> GSGGGDDMSNAGDFLNDNAVEIPSFSKGIINDDEDDEDLMMASGRPRQRSHILEDDENSVDISMLKTGSSLLKEEEEDGQEGSIHNLPLVTSQRPFYDGPMPTPRQKPFQSGSTPLHLTHRFMVWNSIGIIRCYNDEQDNAIDVEFHDTSIHHATHLSNTLNYTIADLSHEAILLACESTDELASKLHCLHFSSWDSSKEWIIDLPQNEDIEAICLGQGWAAAATSALLLRLFTIGGVQKEVFSLAGPVVSMAGHGEQLFIVYHRGTGFDGDQCLGVQLLELGKKKKQILHGDPLPLTRKSYLAWIGFSAEGTPCYVDSEGIVRMLNRGLGNTWTPICNTREHCKGKSDHYWVVGIHENPQQLRCIPCKGSRFPPTLPRPAVAILSFKLPYCQIATEKGQMEEQFWRSVIFHNHLDYLAKNGYEYEESTKNQATKEQQELLMKMLALSCKLEREFRCVELADLMTQNAVNLAIKYASRSRKLILAQKLSELAVEKAAELTAT

Ctf4 orthologues have been identified in various eukaryotic organisms, including fission yeast (Mcl1), Drosophila (Ctf4) and humans (acidic and nucleoplasmic DNA-binding protein; AND-1), suggesting that its functional role has been conserved throughout evolution. AND-1 clearly shares some or possibly all the functions of its yeast counterpart in maintaining genome stability and establishing sister chromatid cohesion. This is a likely consequence of its sequence similarity with Ctf4 (21% identity and 36% similarity over 722 out of 1129 aligned residues) and their shared domain structure, comprising an N-terminal β-propeller domain and a C-terminal SepB domain, the latter being responsible for trimerization and for interactions with proteins harbouring a Ctf4-interacting peptide (CIP) motif. Here, we show that the SepB domain of AND-1 is a structural orthologue of yeast Ctf4, that it exists in a trimeric form and that it binds to Pol α/primase, like its yeast orthologue Ctf4.

To investigate further the structural basis for the interaction of AND-1 with Pol α, we determined the crystal structure of amino acids 329–826 of human AND-1, comprising its SepB domain, which correspond to the region of Ctf4 (Ctf4CTD) that we had previously characterized. Despite the low sequence identity (17%, based on structure superposition), the AND-1 SepB structure bears a remarkable resemblance to that of yeast Ctf4CTD, with the same tertiary structure comprising a six-bladed β-propeller fused to a C-terminal bundle of five α-helices, and an RMSD value of 1.8 Å over 305 Cα positions. In the AND-1 structure, the trimeric arrangement of protomers seen for Ctf4 arises from crystallographic symmetry, and it was confirmed by size-exclusion chromatography multi-angle laser light scattering measurements. Indeed, inspection of the putative binding site for its client proteins, based on structural homology with the Ctf4CTD structure, highlights a solvent-exposed hydrophobic patch formed by M766, A770, A792, L795 and Y799. The pulldown experiments showed a clear interaction of Pol α148–171 with AND-1336–826, which was not observed for the double alanine mutant. Together, these findings indicate that AND-1336–826 is a structural and oligomeric analogue of Ctf4CTD, and that it interacts with its client protein Pol α using the same molecular mechanism. The resulting dissociation constant of 39 µM showed that the interaction of AND-1 with Pol α CIP is surprisingly weak, and prompted us to ask whether other regions of AND-1 and Pol α/primase contribute to their reciprocal association. Crystals of AND-1 329–826 were grown at 9 mg ml−1 using the hanging-drop vapour diffusion technique, in 0.1 MHEPES pH 7.0, 1.1 M di-sodium malonate and 0.5% (v/v) Jeffamine ED-2003, supplemented with 0.36–0.42 M sulfobetaine NDSB-195. The protein crystallized in the cubic space group F 4 3 2 with unit cell dimensions of a = b = c = 249.72 Å and one AND-1 protomer per asymmetric unit.>LVATTSSKIYDNKNQLIADLGSER[2x];>SASNYPAYMDNYLKEVINQVEEETGYNLLTTGMDVYTNVDQEAQKHLWDIYNTDEYVAYPDDELQVASTIVDVSNGKVIAQLGARHQSSNVSFGINQAVETNRDWGSTMKPITDYAPALEYGVYDSTATIVHDEPYNYPGTNTPVYNWDRGYFGNITLQYALQQSRNVPAVETLNKVGLNRAKTFLNGLGIDYPSIHYSNAISSNTTESDKKYGASSEKMAAAYAAFANGGTYYKPMYIHKVVFSDGSEKEFSNVGTRAMKETTAYMMTDMMKTVLSYGTGQNAYLAWLPQAGKTGTSNYTDEEIENHIKTSQFVAPDELFAGYTRKYSMAVWTGYSNR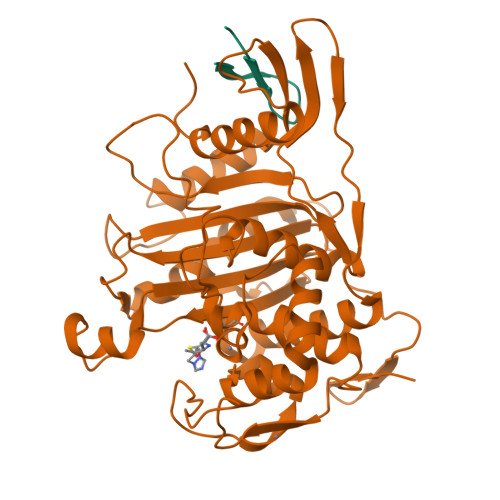LTPLVGNGLTVAAKVYRSMMTYLSEGSNPEDWNIPEGLYRNGEFVFKNGAR[2x]17-oxoandrost-5-en-3beta-yl 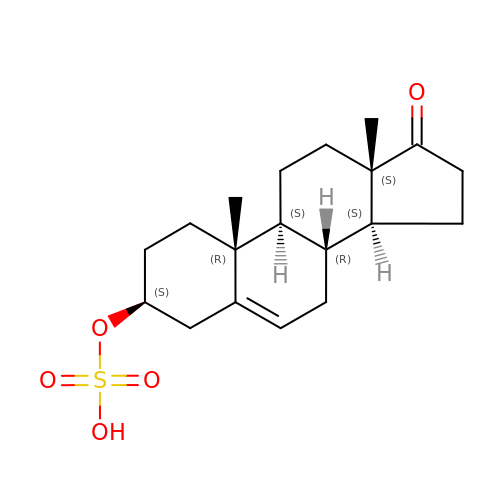hydrogen sulfate | C19 H28 O5 S | CZWCKYRVOZZJNM-USOAJAOKSA-N N-[3-[(3S)-1-azanyl-5-fluoranyl-3-methyl-4H-2,6-naphthyridin-3-yl]-4-fluoranyl-phenyl]-5-cyano-3-methyl-pyridine-2-carboxamide | C23 H18 F2 N6 O | 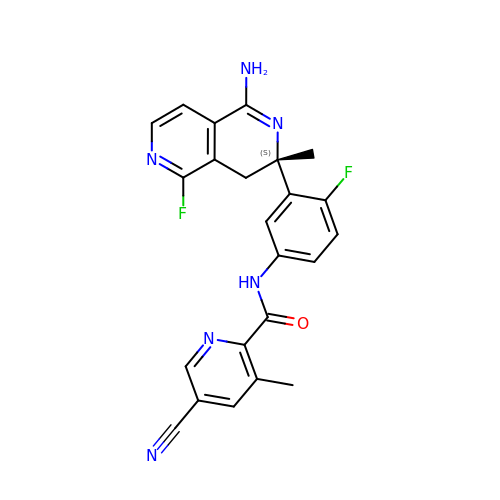UOHLPZVSOSMODJ-QHCPKHFHSA-N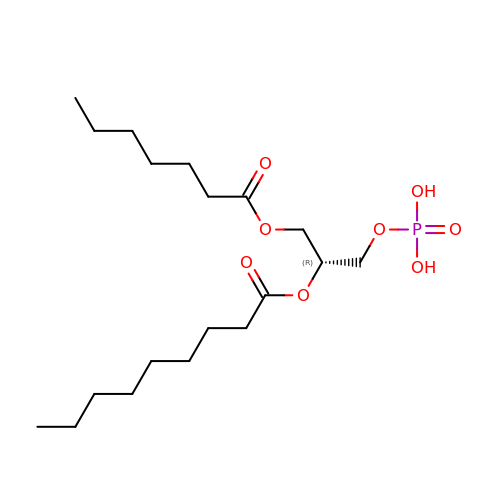[(2R)-2-heptanoyloxy-3-phosphonooxy-propyl] nonanoate | C19 H37 O8 P | XKPYMIOWFWFMRM-QGZVFWFLSA-N>STKKKPLTQEQLEDARRLKAIYEKKKNELGLSQESVADKMGMGQSGVGALFNGINALNAYNAALLAKILKVSVEEFSPSIAREIYEMYEA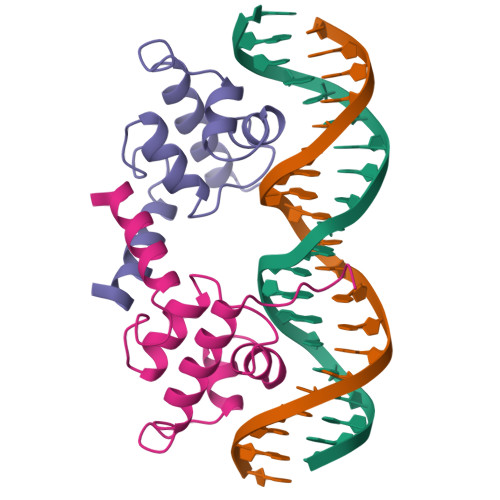VS[2x]>[10x]DYKDDDDKLHSQANLMRLKSDLFNRSPMYPGPTKDDPLTVYLSFSLLDIVKADSSTNEVDLVYWEQQSWKLNSLMWDPN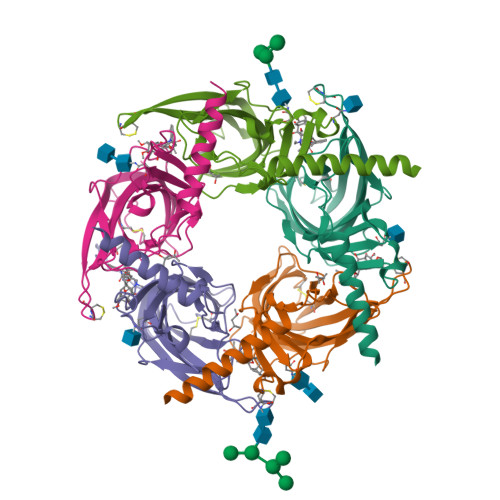EYGNITDFRTSAADIWTPDITAYSSTRPVQVLSPQNALVNSSGHVQYLPAQRLSFMCDPTGVDSEEGATCAVKFGSWSYGGWEIDLKTDTDQVDLSSYYASSKYEILSATQTRQVQHYSCCPEPYIDVNLVVKFRERRAGNGFFRNLFDSR>MTLEQAIERAGTKHGNKGWEAALSAIEMANLFKSLRGTGGSGSSMEIYEGKLTAEGLRFGIVASRFNHALVDRLVEGAIDCIVRHGGREEDITLVRVPGSWEIPVAAGELARKEDIDAVIAIGVLIRGATPHFDYIASEVSKGLANLSLELRKPITFGVITAD[120x]

As such, we found that a circularly permuted variant of a cage-forming enzyme, Aquifex aeolicus lumazine synthase, cpAaLS, assembles into a variety of hollow spherical and cylindrical structures in response to changes in ionic strength. Cryogenic electron microscopy revealed that these structures are composed entirely of pentameric subunits, and the dramatic cage-to-tube transformation is attributed to the moderately hindered 3-fold symmetry interaction and the imparted torsion angle of the building blocks, where both mechanisms are mediated by an α-helix domain that is untethered from the native position by circular permutation. While the wild-type protein, AaLS-wt, self-assembles into a ∼ 16 nm dodecahedral structure composed of 60 identical monomers,35 the negatively supercharged variants AaLS-neg and AaLS-13 adopt expanded 360- and 720-mer assemblies, respectively, constructed entirely from pentameric capsomers. Moreover, a circularly permuted variant of AaLS, cpAaLS(119), forms not only ∼24 nm and ∼28 nm expanded spherical cages, but also straight ∼24 nm-wide tubes of variable length. We previously designed two circularly permuted variants of AaLS and confirmed that their morphologies depend on the positions of the newly generated N- and C-termini. The native terminal amino acids were connected via an octapeptide linker using genetic fusion and new sequence termini were introduced either between residues 84 and 85 or 119 and 120, yielding cpAaLS(84) or cpAaLS(119), respectively.

In 1 M NaCl, the tubes remained a 2% minority, while the ∼28 nm cage constituted ∼30% and the smaller ∼24 nm cages dominated at ∼59%. For example, with 1 M NaCl at pH 8.5, 8.0, and 7.5, the proportion of 24 nm spherical cages was 9%, 59%, and 74%, respectively. The 24 and 28 nm spherical cages are composed of 24- and 36-pentamers, respectively, and both have tetrahedral symmetry, resembling those formed by the previously engineered AaLS variants, NC-1 and AaLS-neg. In contrast, cpAaLS(119) assemblies are non-quasi-equivalent, where at least one interface of the pentameric subunits remains uncontacted. While the number of pentamer–pentamer contacts remains 0 or 1 without NaCl at pH 8.5, judged by the 2D-averaged cryo-EM images, the mean contact number per pentamer increases to 3, 3.7, and 4 in the tubular, 28 nm-, and 24 nm spherical cages, respectively. The bonding network observed at the 2-fold symmetry interface of AaLS-wt is approximately preserved for all the interacting pentamers in the cpAaLS(119) assemblies. In marked contrast, the (pseudo) 3-fold symmetrical interaction interface of cpAaLS(119) assemblies lacks cryoEM density corresponding to the N-terminal α-helix(120–131). This finding suggests that the α-helix is unable to form the native-like hydrophobic cluster, likely due to the disconnection of residues 119 and 120 for circular permutation.> MSSDEEEARELIERAKEAAERAQEAAERTGDPRVRELARELKRLAQEAAEEVKRDPSSSDVNEALKLIVEAIEAAVRALEAAERTGDPEVRELARELVRLAVEAAEEVQRNPSSSDVNEALKLIVEAIEAAV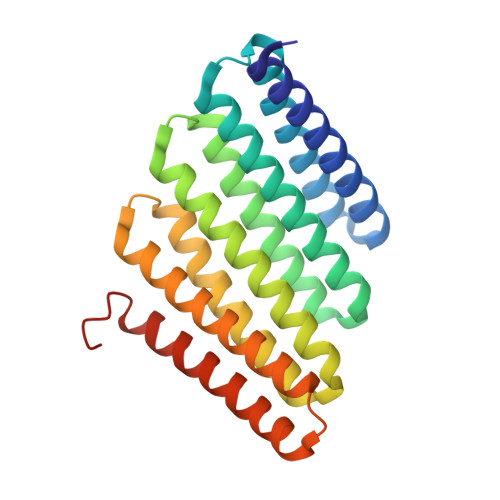RALEAAERTGDPEVRELARELVRLAVEAAEEVQRNPSSEEVNEALKKIVKAIQEAVESLREAEESGDPEKREKARERVREAVERAEEVQRDPSGWLEHHHHHH> XD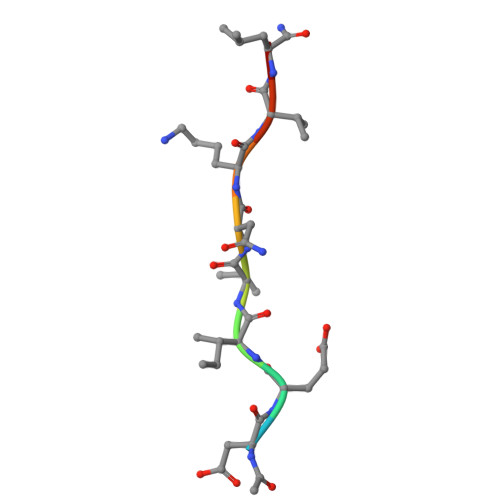EIVNKVLX Here, we characterized E. limosum Tub, a tungsten storage protein. Tub has a sub-nanomolar affinity for tungstate and contains a single TOBE domain first characterized in a molybdate storage protein. Crystal structures revealed Tub assembles as a hexamer composed of a trimer of dimers, capable of binding eight tungstate oxyanions at two distinct binding sites located at inter-subunit interfaces. Tub enables E. limosum to accumulate W and then supplies W for two tungstoenzymes needed for conversion of lactate to SCFAs.

Additional X-ray crystal structures of rTub occupied with varying amounts of W revealed that tungstate accesses the internal type-2 binding sites through tunnels that are closed after binding. With seven tungstate bound, all six type-2 binding sites are occupied and one type-1 site. Based on the occupancy and B-factor statistics, a binding model of tungstate to Tub is proposed. Tungstate simultaneously binds to type-1 and type-2 sites indicating random binding, except for the final binding site located within the trimer center.

>MKLSARNQLAGKVVSIKEGAVNGIVVLDIGGGNQISSTISMDSIRELGLQVGSDAYAVIKATSVMIGIDDWS[6x]>[2x]MKIRDLLKARRGPLFSFEFFPPKDPEGEEALFRTLEELKAFRPAFVSITYGAMGSTRERSVAWAQRIQSLGLNPLAHLTVAGQSRKEVAEVLHRFVESGVENLLALRGDPPRGERVFRPHPEGFRYAAELVALIRERYGDRVSVGGAAYPEGHPESESLEADLRHFKAKVEAGLDFAITQLFFNNAHYFGFLERARRAGIGIPILPGIMPVTSYRQLRRFTEVCGASIPGPLLAKLERHQDDPKAVLEIGVEHAVRQVAELLEAGVEGVHFYTLNKSPATRMVLERLGLRPASGQP

The flavoprotein methylenetetrahydrofolate reductase (MTHFR) catalyzes the reduction of N5, N10-methylenetetrahydrofolate (CH2-H4folate) to N5-methyltetrahydrofolate (CH3-H4folate), committing a methyl group from the folate cycle to the methionine one. MTHFR requires flavin adenine nucleotide (FAD) as a noncovalently bound cofactor, which acts as an intermediary electron shuttle. All MTHFRs share a highly conserved catalytic domain, despite varying oligomerization states, such as a dimer in Thermus thermophilus HB8 (tMTHFR) versus a tetramer in Escherichia coli (eMTHFR). All MTHFR catalytic domains share the same β8α8 barrel topology, a typical triose phosphate isomerase barrel structure.

Here, we report the structure of a tMTHFR holodimer in complex with an N5-formyltetrahydrofolate (CHO-H4folate) substrate analog. We found that in the presence of CHO-H4folate, the tMTHFR dimer adopts the same intermolecular interface as the tMTHFR with half-FAD occupancy (dimer mode 1), despite the presence of FAD in both active sites. In the ternary complex of tMTHFR with FAD and CHO-H4folate bound (referred to as “tMTHFR•CHO-H4folate” in this paper), we observe that the folate pterin ring is stacked against the si-face of the FAD isoalloxazine ring. However, in the tMTHFR•CHO-H4folate structure, the upper side of the PABA ring is occupied by Arg219 with Phe220 (corresponding to Phe223 in eMTHFR) relocating but still engaging, albeit from the side rather than from above, with the PABA ring. As a result, a unique PABA pocket is observed in the tMTHFR•CHO-H4folate structure, in where Phe20 and Arg219 now sandwich and enclose the PABA moiety. In tMTHFR•CHO-H4folate, where L4 adopts an open conformation, in addition to the water (water 3) that bridges Asp109 and the FAD N1-C2=O, there is an additional water molecule (water 2) that is inserted between the folate and FAD; the hydrogen-bonding network between FAD and folate is thus disrupted, and the additional water is hydrogen bonded to C4-O folate and the O atom of the FAD N1-C2=O moiety. As a result, the distance between the N1 of FAD and Asp109 increases to 5.3 Å. The repositioning of Thr49 in the tMTHFR•CHO-H4folate structure is of particular note. The Thr49 hydroxyl group hydrogen bonds with the Glu18 side chain in the tMTHFR•CHO-H4folate structure, a residue whose polarity, as previously mentioned, is essential for catalysis As a result of the Thr49 relocation and its hydrogen bonding with Glu18, an extended quartet is now formed in the active site that also includes His270 and Ser16. Indeed, the distance between N5-C of folate and N5 of FAD in the eMTHFR•CH3-H4folate structure is 3.3 Å (14), while that in the tMTHFR•CHO-H4folate structure is 3.8 Å in one monomer and 4.0 Å in the other. The longer distance observed between folate N5-C and FAD N5 in the tMTHFR•CHO-H4folate structure indicates that the ligands and active site residues are not in an arrangement (as) conducive to hydride transfer.>NTQLMGERIRARRK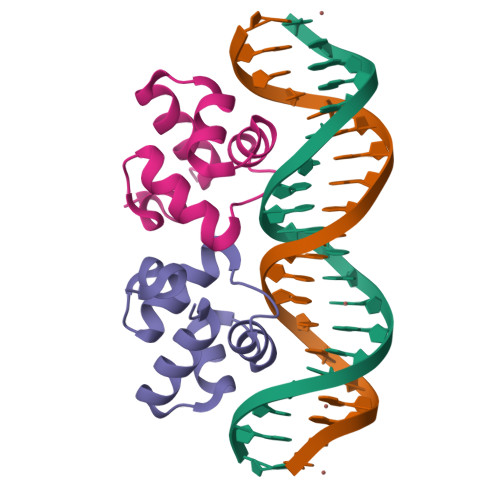KLKIRQAALGKMVGVSNVAISQWERSETEPNGENLLALSKALQCSPDYLLKGD[2x]> MAARRAPISRRDRPAKPALSRRWIVDTAVALMRAEGLEKVTMRRLAQELDTGPASLYVYVANTAELHAAVLDALLGEVDLTGAGAEEDWREQLRAVLTSYTLVLFAHPQLARSALVARPSGENYLRLVERVLELL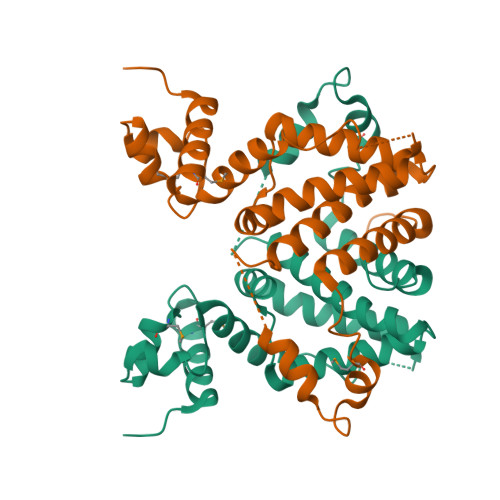ARSGAPGAQVAWGVDKLLQDATATAAEQATQEHDPASHEDWSATVRALRDADEATHPAIASHMPLLVAGSAHDRLRWSFDVLVNGITRTPVPGPARGAAGLEHHHHHH> VKKT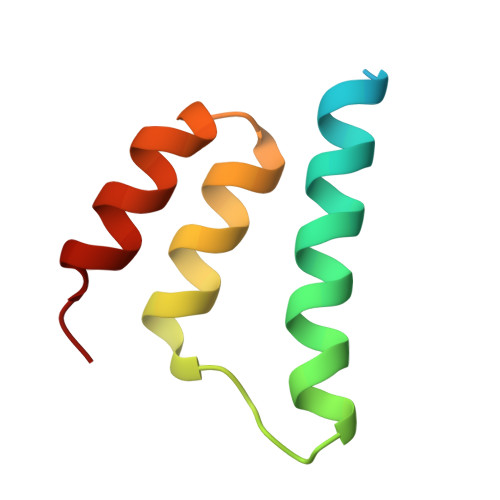TDHSTSLTSEELQKRREAVDAAISTHAIEGITLHSKTLEILEGYAKGEYSLEEFNTLMDNATL> MSYLNLRLYQRNTQCLHIRKHRLAGFFVRLFVACAFAAQASLSSAELYFNPRFLADDPQAVADLSRFENGQELPPGTYRVDIYLNNGYMATRDVTFNTGDSEQGIVPCLTRAQLASMGLNTASVAGMNLLADDACVPLTTMVQDATAHLDVGQQRLNLTIPQAFMSNRARGYIPPELWDPGINAGLLNYNFSGNSVQNRIGGNSHYAYLNLQSGLNIGAWRLRDNTTWSYNSSDRSSGSKNKWQHINTWLERDIIPLRSRLTLGDGYTQGDIFDGINFRGAQLASDDNMLPDSQRGFAPVIHGIARGTAQVTIKQNGYDIYNSTVPPGPFTINDIYAAGNSGDLQVTIKEADGSTQIFTVPYSSVPLLQREGHTRYSITAGEYRSGNAQQEKPRFFQSTLLHGLPAGWTIYGGTQLADRYRAFNFGIGKNMGALGALSVDMTQANSTLPDDSQHDGQSVRFL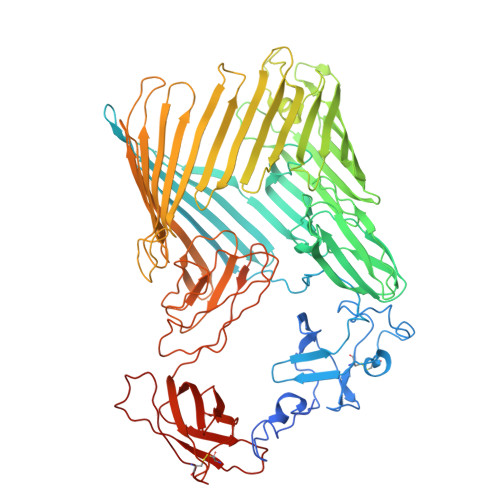YNKSLNESGTNIQLVGYRYSTSGYFNFADTTYSRMNGYNIETQDGVIQVKPKFTDYYNLAYNKRGKLQLTVTQQLGRTSTLYLSGSHQTYWGTSNVDEQFQAGLNTAFEDINWTLSYSLTKNAWQKGRDQMLALNVNIPFSHWLRSDSKSQWRHASASYSMSHDLNGRMTNLAGVYGTLLEDNNLSYSVQTGYAGGGDGNSGSTGYATLNYRGGYGNANIGYSHSDDIKQLYYGVSGGVLAHANGVTLGQPLNDTVVLVKAPGAKDAKVENQTGVRTDWRGYAVLPYATEYRENRVALDTNTLADNVDLDNAVANVVPTRGAIVRAEFKARVGIKLLMTLTHNNKPLPFGAMVTSESSQSSGIVADNGQVYLSGMPLAGKVQVKWGEEENAHCVANYQLPPESQQQLLTQLSAECRS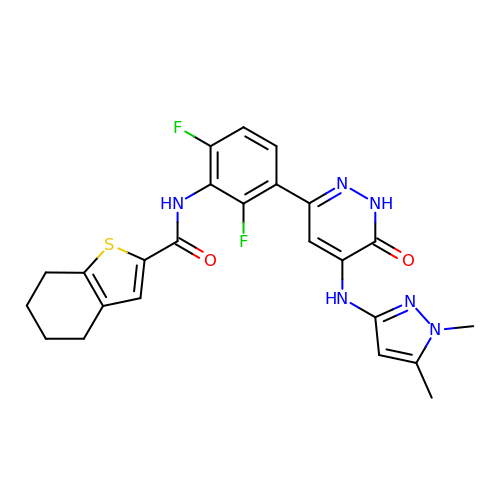N-(3-{5-[(1,5-dimethyl-1H-pyrazol-3-yl)amino]-6-oxo-1,6-dihydropyridazin-3-yl}-2,6-difluorophenyl)-4,5,6,7-tetrahydro-1-benzothiophene-2-carboxamide | C24 H22 F2 N6 O2 S | ABEMEXKJBCGDPX-UHFFFAOYSA-N> SELEKA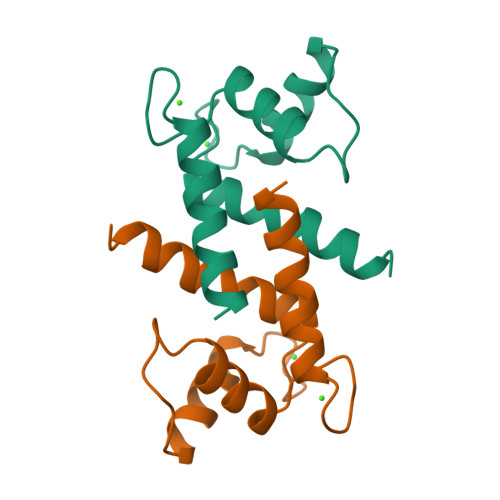VVALIDVFHQYSGREGDKHKLKKSELKELINNELSHFLEEIKEQEVVDKVMETLDSDGDGECDFQEFMAFVAMITTACHEFF> SDSLSKSPENWMSKLDDGKHLTEINIPGSHDSGSFTLKDPVKSVWAKTQDKDYLTQMKSGVRF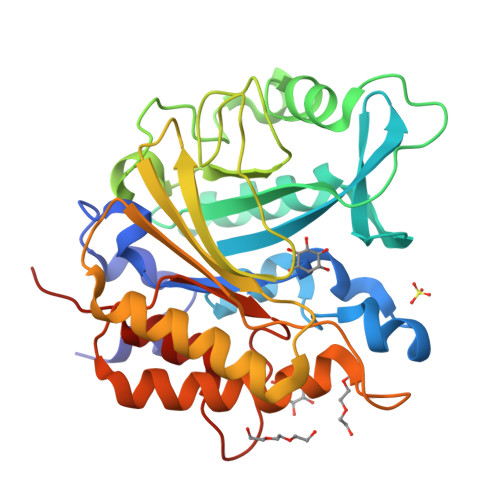FDIRGRASADNMISVHHGMVYLHHELGKFLDDAKYYLSAYPNETIVMSMKKDYDSDSKVTKTFEEIFREYYYNNPQYQNLFYTGSNANPTLKETKGKIVLFNRMGGTYIKSGYGADTSGIQWADNATFETKINNGSLNLKVQDEYKDYYDKKVEAVKNLLAKAKTDSNKDNVYVNFLSVASGGSAFNSTYNYASYINPEIAKTIKANGKARTGWLIVDYAGYTWPGYDDIVSEIIDSNKLEHHHHHH{4-[(2-{[(4-tert-butylphenyl)methyl]sulfanyl}acetamido)methyl]-1H-1,2,3-triazol-1-yl}acetic acid | C18 H24 N4 O3 S | 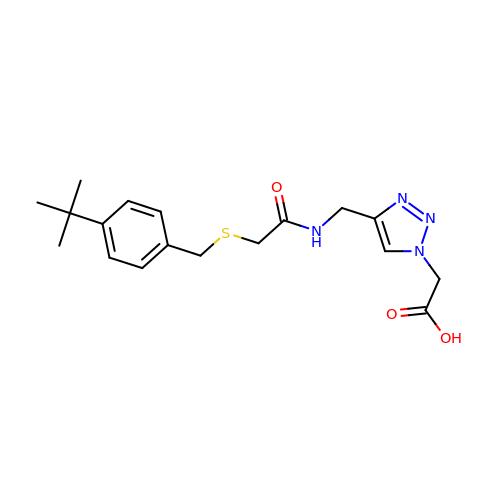HCTZVVOCYIXIAH-UHFFFAOYSA-N3-[2-morpholin-4-yl-6-(pyridin-3-ylamino)pyrimidin-4-yl]phenol | C19 H19 N5 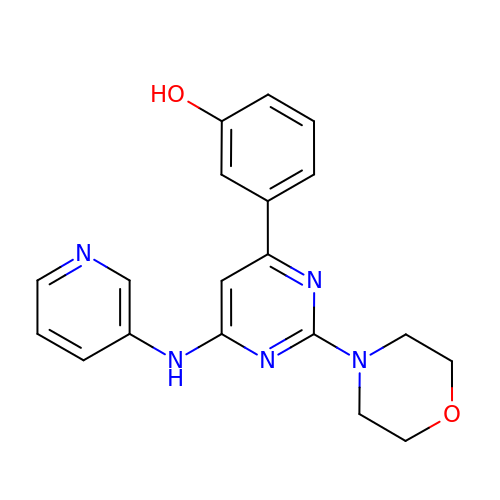O2 | VPAXYWZGMCIWNR-UHFFFAOYSA-N>[8x]MTQPMPGKPAEDAENELDIRGLFRTLWAGKLWIIGMGLAFALIALAYTFFARQEWSSTAITDRPTVNMLGGYYSQQQFLRNLDVRSNMASADQPSVMDEAYKEFVMQLASWDTRREFWLQTDYYKQRMVGNSKADAALLDEMINNIQFIPGDFTRAVNDSVKLIAETAPDANNLLRQYVAFASQRAASHLNDELKGAWAARTIQMKAQVKRQEEVAKAIYDRRMNSIEQALKIAEQHNIS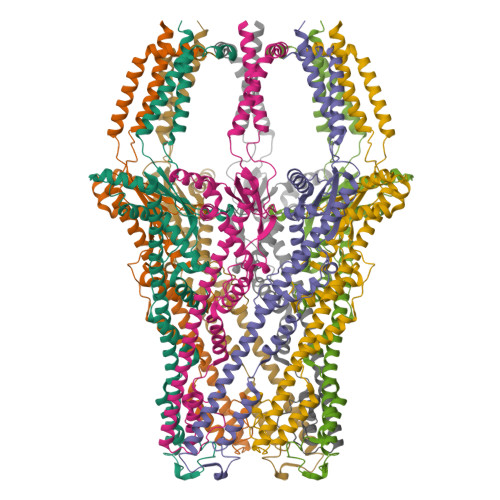RSATDVPAEELPDSEMFLLGRPMLQAELENLQAVGPAFDLDYDQNRAMLNTLNVGPTLDPRFQTYRYLRTPEEPVKRDSPRRAFLMIMWGIVGGLIGAGVALTRRCSKEFRVPGSHHHHHHHH>[180x]SNIMSTSGTGKMTRAQRRAAARRNR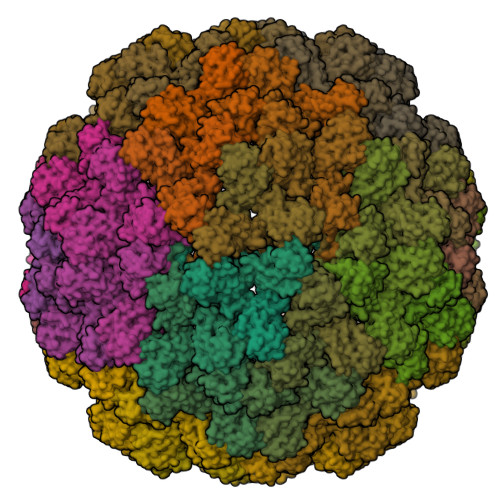RTAGVQPVIVEPIAAGQGKAIKAIAGYSISKWEASSDAITAKATNAMSITLPHELSSEKNKELKVGRVLLWLGLLPSVAGRIKACVAEKQAQAEAAFQVALAVADSSKEVVAAMYTDAFRGATLGDLLNLQIYLYASEAVPAKAVVVHLEVEHVRPTFDDFFTPVYK>SAHTLRLDESHVHLVDSKDKFYAMLSDLCRQSMIAFASEWKPTFGGANEVSLIQLATWDDVYMIDVMVSQLEPLDWAALAKNVFNRDDVLKLSFAPSTDISMFQKALPSFNVMYSSQSTSAILDLQLLWRHVERFDSFRFPYHEESVNQNLANLVRLCLGKKLDKSNQFSNWAQRPLRKEQ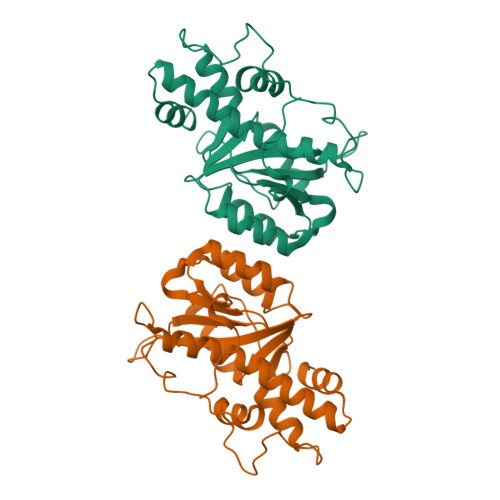LRYAALDAFCLLEIYDAIEKQLTHIQLDPNEILNALLNDVRPPSDS[2x]>[4x]APQQINDIVHRTITPLIEQQKIPGMA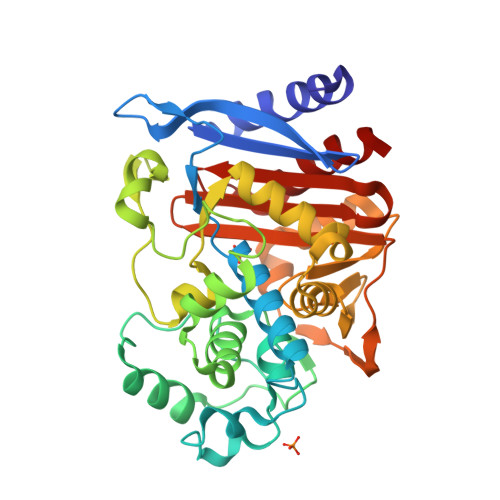VAVIYQGKPYYFTWGYADIAKKQPVTQQTLFELGSVSKTFTGVLGGDAIARGEIKLSDPTTKYWPELTAKQWNGITLLHLATYTAGGLPLQVPDEVKSSSDLLRFYQNWQPAWAPGTQRLYAGSSIGLFGALAVKPSGLSFEQAMQTRVFQPLKLNHTWINVPPAEEKNYAWGYREGKAVHVSPGALDAEAYGVKSTIEDMARWVQSNLKPLDINEKTLQQGIQLAQSRYWQTGDMYQGLGWEMLDWPVNPDSIINGSDNKIALAARPVKAITPPTPAVRASWVHKTGATGGFGSYVAFIPEKELGIVMLANKNYPNPARVDAAWQILNALQ{4-[2-BENZYL-3-METHOXY-2-(METHOXYCARBONYL)-3-OXOPROPYL]PHENYL}SULFAMIC ACID | C19 H21 N O7 S | 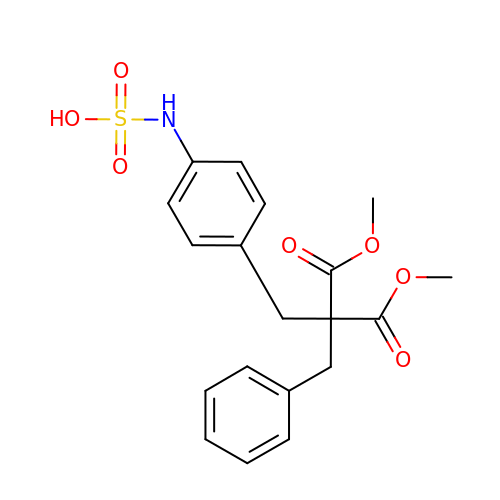SUACYXRSGYYBGT-UHFFFAOYSA-N>[2x]PQKLFGEVTSPLFPKPYPNNFETTTVITVPTGYRVKLVFQQFDLEPSEGCFYDYVKISADKKS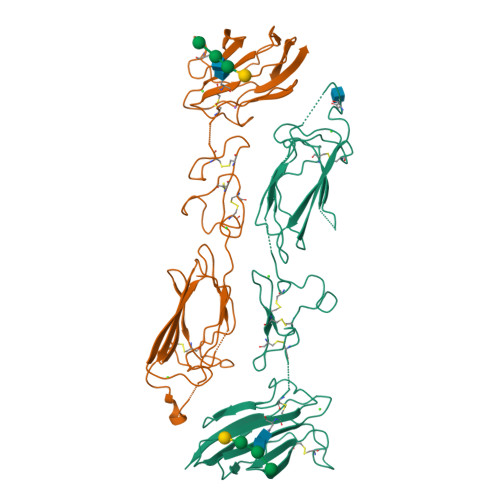LGRFCGQLGSPLGNPPGKKEFMSQGNKMLLTFHTDFSNEENGTIMFYKGFLAYYQAVDLDECASRSKSGEEDPQPQCQHLCHNYVGGYFCSCRPGYELQEDTHSCQAECSSELYTEASGYISSLEYPRSYPPDLRCNYSIRVERGLTLHLKFLEPFDIDDHQQVHCPYDQLQIYANGKNIGEFCGKQRPPDLDTSSNAVDLLFFTDESGDSRGWKLRYTTEI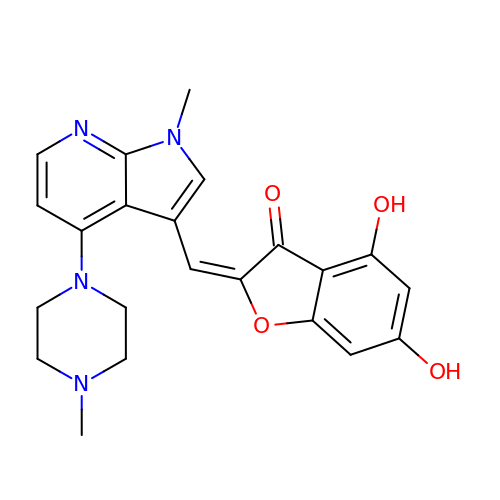(2Z)-4,6-dihydroxy-2-{[1-methyl-4-(4-methylpiperazin-1-yl)-1H-pyrrolo[2,3-b]pyridin-3-yl]methylidene}-1-benzofuran-3(2H)-one | C22 H22 N4 O4 | RLZIWQDVHJTWEF-NVMNQCDNSA-N> PARPPKP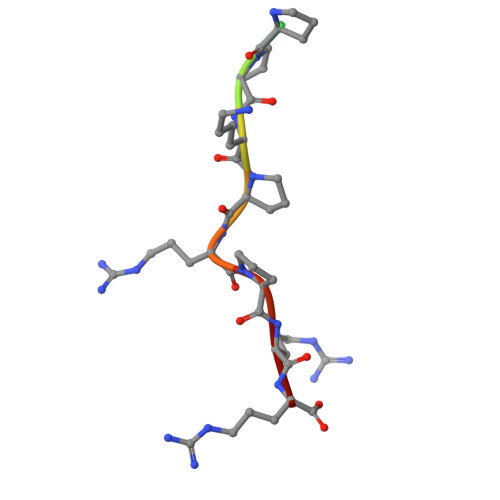RPRR> AQ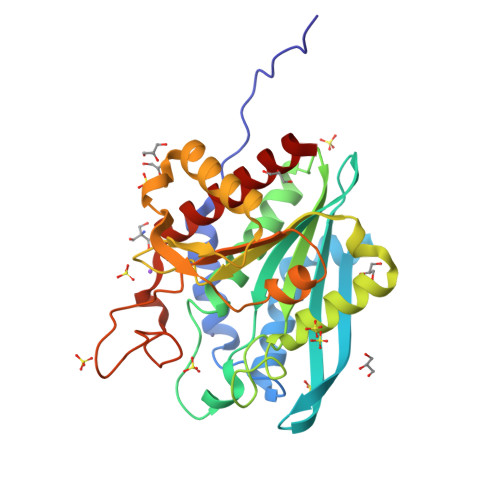KAPAQNSPARFNGQAAYNLTRQYIAAAPKRWVGSPGHAKAEAFIKDHFKPEIAQGRFETDRFTAGTPAGLLEMRNYIVRYPGKKDGVIVLATHYETNYPLRDINFVGANDGGSTTALLIEMGNYLRAHPPQGYSIWLVFDDGEEAIQSWSATDSLYGTRHLAAKWSQDGTLKKIKAFLLADMIGDKDLNIDRDANSTPWLLDMLKQAAKNTGHSAYVFKNSTAVEDDHLPFAKRGVPVLDIIDIDYGPRTFSMPDGYHHTAEDTLDKISAHSLQIAGDLFLEMIRLINQRG> S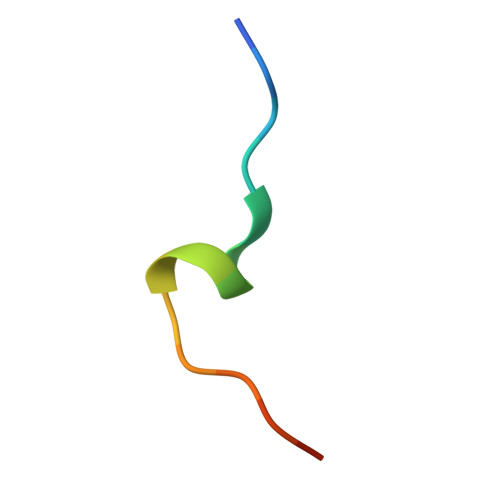TQGRLDDFFKVTGSL Enteropathogenic *E. coli* (EPEC) O127:H6 encodes an additional, tripartite TA module, *hipBST*, for which the HipT toxin was shown to specifically target tryptophanyl-tRNA synthetase, TrpS. Surprisingly, the function as antitoxin has been taken over by the third protein, HipS, but the molecular details of how activity of HipT is controlled remain poorly understood. Here, we show that HipBST is markedly different from HipBA and that the unique HipS protein, which is homologous to the N-terminal subdomain of HipA, has evolved to function as antitoxin by breaking the kinase active site. We also show how auto-phosphorylation at two conserved sites in the kinase toxin serve to dually regulate binding of HipS and kinase activity.

To understand the individual roles of the two autophosphorylation positions, we next determined crystal structures of two HipBST complexes with HipT serine residues mutated to alanine individually: HipBST^S57A^ (2.4 Å, [Table tblS1]) and HipBST^S59A^ (3.4 Å). The phosphate groups on Ser57 (in S59A) and Ser59 (in S57A) are shown in orange and relevant nearby residues are highlighted. **b.** Close-up of the HipT active site as observed for the S57A mutant with relevant active site residues shown as sticks. In both structures, however, the Gly-rich loop maintains its outward conformation, incompatible with ATP binding, suggesting that HipT is inactive. Intriguingly, the phosphoryl group of P-Ser57 overlaps structurally with that of phosphorylated Ser147 in HipA_So_, which corresponds to HipA_Ec_ Ser150 at the sequence level ([Fig figS4]**, bottom**). Here, we observed a marked difference in migration between HipT from wildtype HipBST, HipBST^S59A^, and HipBST^S57A^ confirming that HipT^S57A^ is predominantly phosphorylated while HipT^S59A^ is only partially modified, consistent with the crystal structures. In summary, we conclude that the conformation of the HipT active site loop (Gly-rich loop) inside the HipBST complex is independent of the autophosphorylation state. Taken together, we conclude that HipT autophosphorylation at Ser57 prevents HipS inhibition and does not prevent phosphorylation of the target, TrpS. Autophosphorylation at Ser 57 severely reduces HipS binding, thereby prolonging the growth inhibitory effect of HipT by keeping the kinase active and preventing full transcriptional repression. Another question raised by the structures is how HipS can be bound in the complex with Ser57 in its phosphorylated state if this serves to block HipS binding? In this context, it is important to note, however, that only a minor fraction of the purified complex is phosphorylated ([Fig fig4]), confirming that if HipT (Ser57-P) binds to HipS at all, it probably binds very poorly.

>ICSGPQNLAQELKAIGDQLQELQKKLIQGPNISQPRPLLTIETPRHLGEQLNARRKELGIDLYTLELQTGISTSTLKRLFKDPEQVKFGSVFAVANVLGVKLCIGE[2x];>HRRVKVLLYGQVVGELSQNDSGFLFQYAHDYHGPAISISLPVAQRQFPSETLHPYFASLAPEGWLRQRYSQIQHRDENDLLGMLIDNGKNLLGAIQILPWEE[2x];>[2x]ANCRILLTPLNERDEQRGYSTQGLKRLSGTAKLNPRLGFTRTQFVQELPRQQKGMSIAGYQPKLQLVLDEGEFRVVDHQGNFILKPSPADFPGLAENEHATMTLMSRLGFDVPVHGLLSFAPQSEEELEYAFVIRRYDRDNKGLPVHQEQLDGAMQITDKYGKTGNDNEQYVSYETLARFLVAHVNDNIAFKIDLFRRIVYAWLLGNNDMHLRNFGLVYSDGLTPALAPVYDFVSVAPYPEYFYSNYLALPLLTREEGGRELAPGFHSDYGEYIGQDFLLLGESMGLAPRLLEKLFQDIRKENAIVMETYEQSFMTQDHIQAVLQCYRHRLGLLHHHHHH>[3x]MAHHHHHHVDDD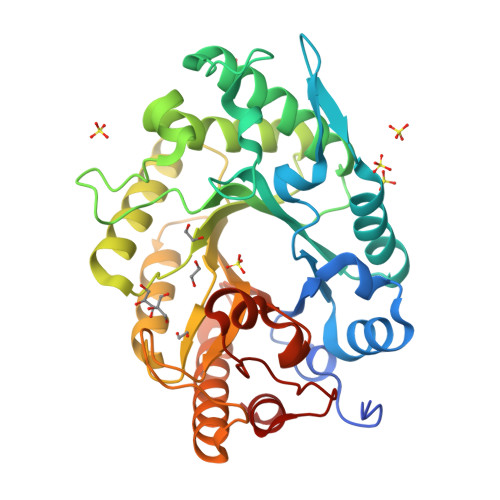DKAPDWSIPSLCESYKDDFIIGVAIPARCLSNDTDKRMVLKHFNSITAENEMKPESLLAGQTSTGLSYRFSTADAFVDFASTNKIGIRGHTLVWHNQTPDWFFKDSNGQRLSKDALLARLKQYIYDVVGRYKGKVYAWDVVNEAIDENQSDGYRRSTWYEICGPEYIEKAFIWAHEADPNAKLFYNDYNTEISKKREFIYNMVKNLKSKGIPIHGIGMQCHINVNWPSVSEIENSIKLFSSIPGIEIHITELDMSLYNYGSSENYSTPPQDLLQKQAQKYKEIFTMLKKYKNVVKSVTFWGLKDDYSWLRSFYGKNDWPLLFFEDYSAKPAYWAVIEA> MEYIKLKVIGQDSSEIHFKVKMTTHLKKLKESYCQRQGVPMN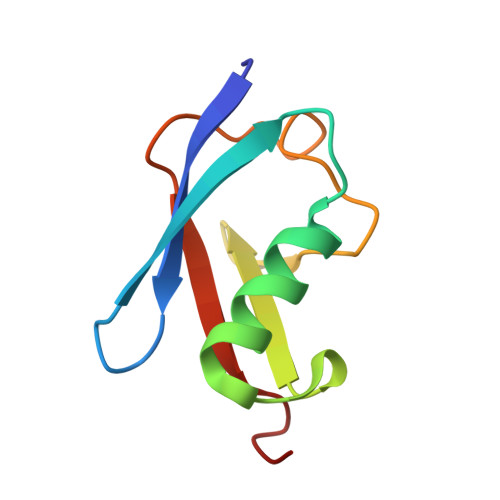SLRFLFEGQRIADNHTPKELGMEEEDVIEVYQEQTGG> GDE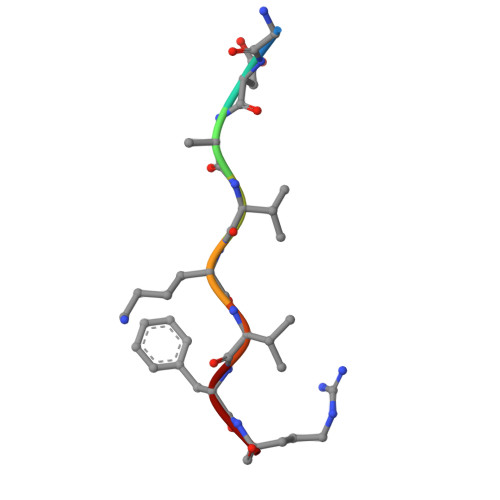VKVFR> GSMKAAYIIKEVQNINSEREGTQIEATSLSQAKRIASKEQCFHGTVM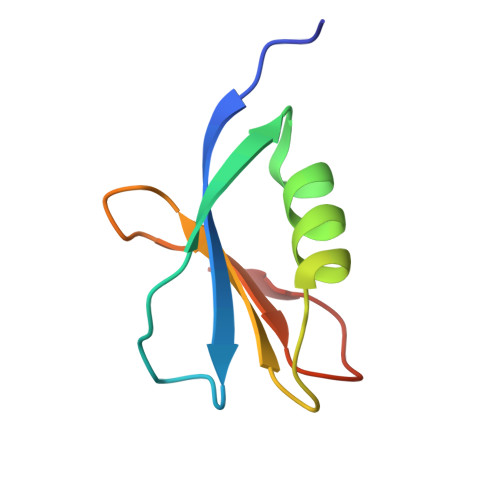RIETVNGLWLAYKEDGKRWVDCQ>GHMNDIQSQIVSRGEEILKRMESQSKASIFSKDFWYGSIMEWSMKNEKFKTNMFRFVDVLPSINSGDEVARHLKEYFSEDGGTLPPVFNVGLGLGSLAPGLMAGAIKKNVMGMAKMFITGESPDEALPVLKKARKNKMTFTVDILGEATLSEKEAQDYSNKYMELVTWLAKDAEKWDEVPQIDRDHEGALPKVNVSVKMTALYSQIKDAAWDESKKILKDRLRPVFRLGMEKGVFVNLDMEQYSVKHLTLEVFTELINEPEFKNYKFFGIVIQAYLRDSFEDVKSLTEFAQKRGTPFWVRLVKGAYWDYETIEAEQRGWPVPVYTNKAESDANYELCAKYLLENIKFIRPAFASHNVRTLAACMLYAEKLNIPKEALEFQMLYGMAEPIKKTIVDMGYRMREYAPVGELIPGMAYLVRRLLENTSNESWLRGKFADNKSMAELLKDPAQGLTPTSPVIPKKPGKFYNEPLLDFAVKADREKMLKALAEAKASLPVNVNIVINNKELQSGKIFDRVNPSQSDQIVGKIQMATTEQAEQAMQAAQTAYKTWKNVPCE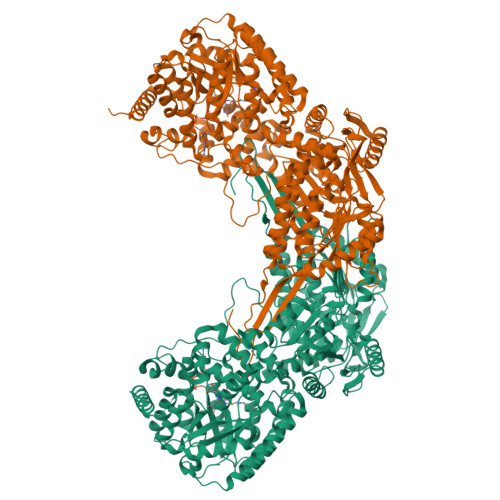QRAALVDKLADIMTRDRFKLIATQVLEVGKPWAEADGDIGEAIDFCRYYARHMRELQKPLRVGGLPGELSHYIYKSRGVTAVIAPWNFPLAILAGMVTAAAVAGNTVVMKPAEQSTVVAWGLMKMIQEAGFPQGVINFLPGYGEEVGEYIVNHKYTTTIAFTGSKAVGLHIMNRAAVVQPGQQHVKRCIIEMGGKNAVIIDNDADLDEAVDGVIYSAFGFSGQKCSAASRVIVLDEVYDRFVDRLVETAKSIEIHPAENPKAYMGPVVDKEAYDRILGTIAEAEKNHKLLFKGSVPGGGFFAPPTIFGDVPGDAKLAQAEIFGPVVAVIRAKNLDQALDIANSTEYALTGGVFSRSPANINRVKEELEVGNLYVNRGITGAMVDRHPFGGFKMSGIGSKTGGPDYLKQYMEPACVTENTLRRGFAPAEE[4x]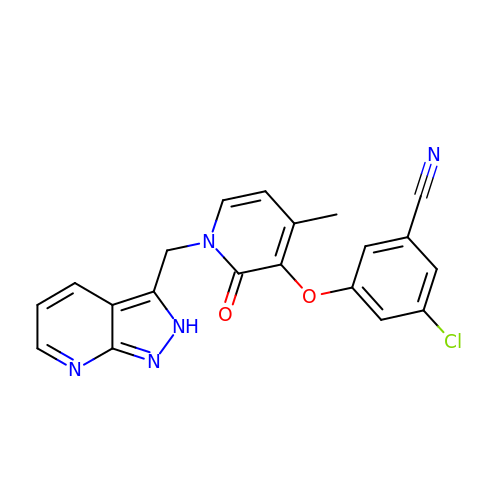3-chloro-5-{[4-methyl-2-oxo-1-(2H-pyrazolo[3,4-b]pyridin-3-ylmethyl)-1,2-dihydropyridin-3-yl]oxy}benzonitrile | C20 H14 Cl N5 O2 | YMRUCOCNLHJFRC-UHFFFAOYSA-N> MISTTISGKRPIEQVDDELLSLTAQQENEEQQQQRKRRRHQFAPMTQFNSNTLDEDSGFRSSSDVATADQDNFLEESPSGYIKKVILRNFMCHEHFELELGSRLNFIVGNNGSGKSAILTAITIGLGAKASETNRGSSLKDLIREGCYSAKIILHLDNSKYGAYQQGIFGNEIIVERIIKRDGPASFSLRSENGKEISNKKKDIQTVVDYFSVPVSNPMCFLSQDAARSFLTASTSQDKYSHFMKGTLLQEITENLLYASAIHDSAQENMALHLENLKSLKAEYEDAKKLLRELNQTSDLNERKMLLQAKSLWIDVAHNTDACKNLENEISGIQQKVDEVTEKIRNRQEKIERYT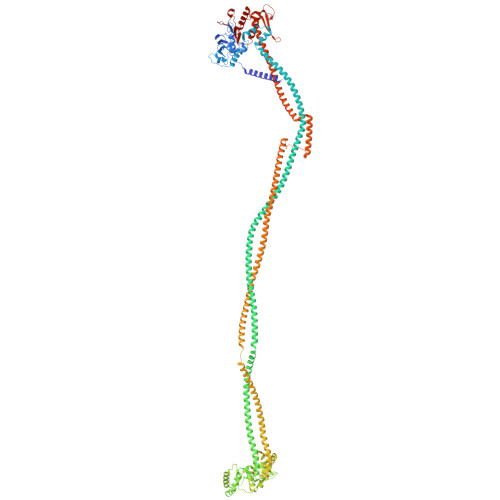SDGTTIEAQIDAKVIYVNEKDSEHQNARELLRDVKSRFEKEKSNQAEAQSNIDQGRKKVDALNKTIAHLEEELTKEMGGDKDQMRQELEQLEKANEKLREVNNSLVVSAQDVKNEERDIQHERESELRTISRSIQNKKVELQNIAKGNDTFLMNFDRNMDRLLRTIEQRKNEFETPAIGPLGSLVTIRKGFEKWTRSIQRAISSSLNAFVVSNPKDNRLFRDIMRSCGIRSNIPIVTYCLSQFDYSKGRAHGNYPTIVDALEFSKPEIECLFVDLSRIERIVLIEDKNEARNFLQRNPVNVNMALSLRDRRSGFQLSGGYRLDTVTYQDKIRLKVNSSSDNGTQYLKDLIEQETKELQNIRDRYEEKLSEVRSRLKEIDGRLKSTKNEMRKTNFRMTELKMNVGKVVDTGILNSKINERKNQEQAIASYEAAKEELGLKIEQIAQEAQPIKEQYDSTKLALVEAQDELQQLKEDINSRQSKIQKYKDDTIYYEDKKKVYLENIKKIEVNVAALKEGIQRQIQNACAFCSKERIENVDLPDTQEEIKRELDKVSRMIQKAEKSLGLSQEEVIALFEKCRNKYKEGQKKYMEIDEALNRLHNSLKARDQNYKNAEKGTCFDADMDFRASLKVRKFSGNLSFIKDTKSLEIYILTTNDEKARNVDTLSGGEKSFSQMALLLATWKPMRSRIIALDEFDVFMDQVNRKIGTTLIVKKLKDIARTQTIIITPQDIGKIADIDSSGVSIHRMRDP>[2x]NSIASCPEEQPHVGNYRLLRTIGKGNFAKVKLARHILTGREVAIKIIDKTQLNPSSLQKLFREVRIMKGLNHPNIVKLFEVIETEKTLYLVMEYASAGEVFDYLVSHGRMKEKEARAKFRQIVSAVHYCHQKNIVHRDLKAENLLLDAEANIK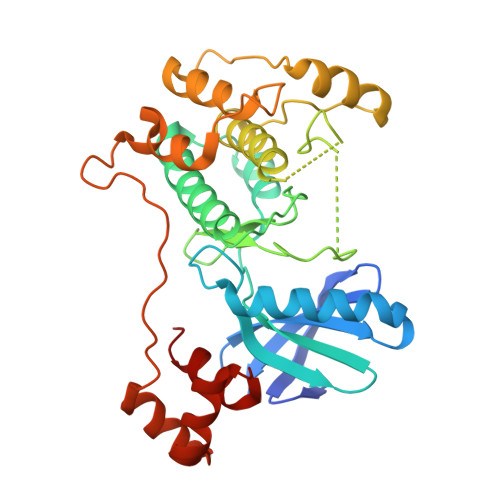IADFGFSNEFTLGSKLDTFCGSPPYAAPELFQGKKYDGPEVDIWSLGVILYTLVSGSLPFDGHNLKELRERVLRGKYRVPFYMSTDCESILRRFLVLNPAKRCTLEQIMKDKWINIGYEGEELKPYTEPEEDFGDTKRIEVMVGMGYTREEIKESLTSQKYNEVTATYLLLGRK> MVKVTYDGVYVMSVKDDVP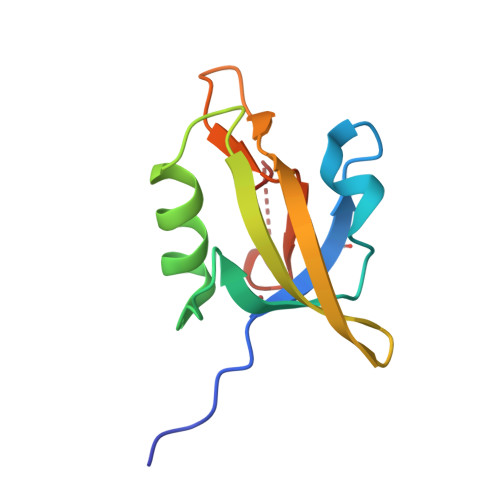AADVLHAGDLITEIDGNAFKSSQEFIDYIHSKKVGDTVKINYKHGDKNEQADIKLTAIDKKGTPGIGITLVDDLEHHHHHH>GHMVPELKQISREEAMRLGPGWSHSCHAMLYAANPGQLFGRIPMRFSVLMQMRFDGLLGFPGGFVDRRFWSLEDGLNRVLGLGLGGLRLTEADYLSSHLTEGPHRVVAHLYARQLTLEQLHAVEISAVHSRDHGLEVLGLVRVPLYTQKDRVGGFPNFLSNAFVSTAKYQLLFALKVLNMMPSEKLAEALASATEKQKKALEKLLPPSS[2x];> GHMNSFVGLRV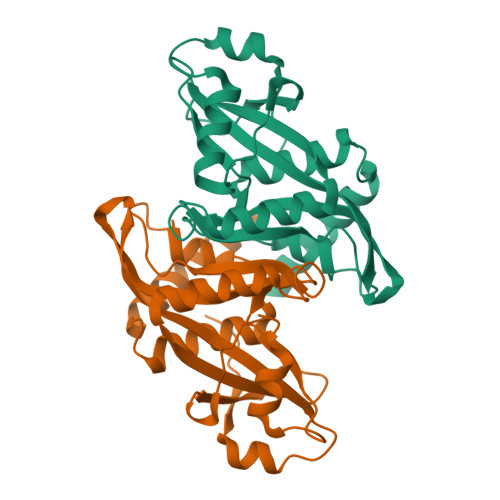VAKWSSNGYFYSGKITRDVGAGKYKLLFDDGYECDVLGKDILLCDPIPLDTEVTALSEDEYFSAGVVKGHRKESGELYYSIEKEGQRKWYKRMAVILSLEQGNRLREQYGLG>[4x]MRNIAEAYFQNMVETATPLEQIILLYDKAIECLERAIEIYDQVNELEKRKEFVENIDRVYDIISALKSFLDHEKGKEIAKNLDTIYTIILNTLV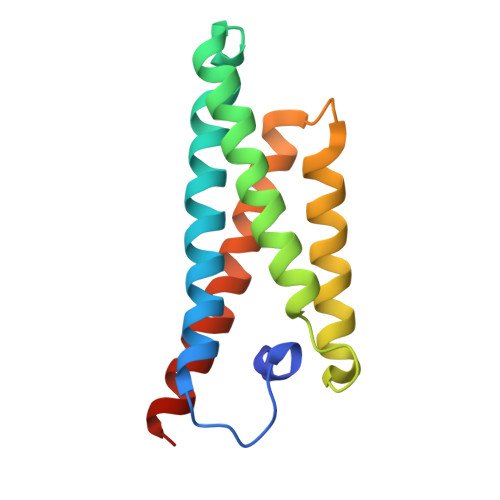KVDKTKEELQKILEILKDLREAWEEVKKKVHHHHHH> MFLYYKMNEVLNVNNGSSINVIKILKTPGPDIIRPGKTYKKKDVFTPKFFKNGNVMYTCNTFSLNVPVNNSIATIDFAEHVNGAVFKIEYNRVNFIAPSLYPISGLGTAVVFDLQKGEKASQ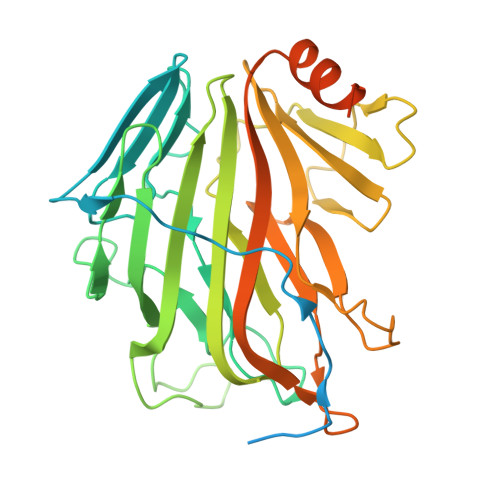RKITEFGNKDIRIADEISDIAADDHSVLITTKLMSESTPGELSRDVVLNGEIATGRINMNTGFVSDIIHTKKISIIDDGIVDYYVKINVPAKYSHGIVEVVSGTFLNDIMIHLVRNKNKWALMDSKMYIVNNTNGFVIAKNPDTAMGVSLLEWPRGAVVFPPYYNFKKFKNVNKWSISQQIASCVNTSVKIPGGEYSWKIRLFFGPIWQVQESINSVKTVPHGNDYMYLYKEEIVKYKYQRNTKRNFHEYDYDYKF>[2x]MQKTLEVWIMPNSPQPAEDFKALVAPFEKAHGVEVKVTVLDWGVAWTKITTAATSGVGPDLTQLGTTWVGAISAMGVLEPVDDVLEALGGEKAYLPAVWRTTRLEGARQATAVPWFSALRA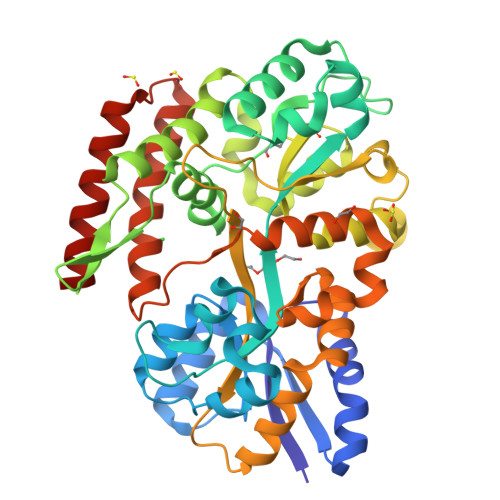FYYRTDALKAAGVNPAEMFASWQGFEAGLARLKASSFRDPETKAPLAPLCTPGKNSWDVLHNAAPWIWGAGGEIVRQAGGRWQSALNSPESLEGLYFFLSLAQKGYVPAESLEKNTAQIEADFQAGKCAVFASGPWMIQRAQVPEAKGGFAERTAAKNLGVAPYPAGPKGRYTFFGGSNLALFNFSKNKPLAKELLKYLGGPEAQVRYAQMTGMLPALRSAWSDPSFQQNPLLRTFIQAAQFGRTYPSLAGWGGVENLAVQHLGMAWDLVAQGRLTREALKDLMDKASAAINQALRHHHHHH>NEDICFIAGIGDTNGYGWGIAKELSKRNVKIIFGIWPPVYNIFMKNYKNGKFDNDMIIDKDKKMNILDMLPFDASFDTANDIDEETKNNKRYNMLQNYTIEDVANLIHQKYGKINMLVHSLANAKEVQKDLLNTSRKGYLDALSKSSYSLISLCKYFVNIMKPQSSIISLTYHASQKVVPGYGGGMSSAKAALESDTRVLAYHLGRNYNIRINTISAGPLASRAATAINKLNNTYENNTNQNKNRNRHDVHNIMNNSGEKEEKKISASQNYTFIDYAIEYSEKYAPLRQKLLSTDI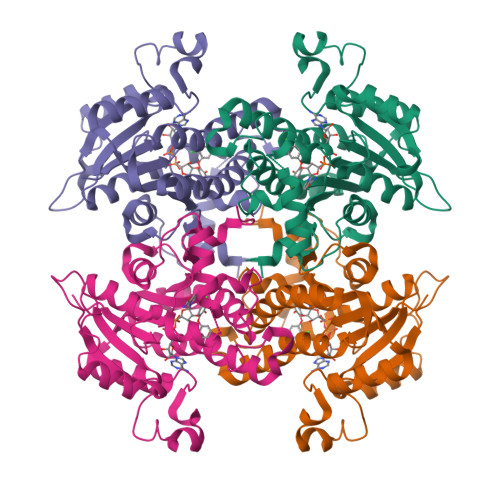GSVASFLLSRESRAITGQTIYVDNGLNIMFLPD[2x]> DRSANTNIAVYWGQNSAGTQESLATYCESSDADIFLLSFLNQFPTLGLNFANACSDTFSDGLLHCTQIAEDIETCQSLGKKVLLSLGGASGSYLFSDDSQAETFAQTLWDTFGEGTGASERPFDSAVVDGFDFDIENNNEVGYSALATKLRTLFAEGTKQYYLSAAPQCPYPDASVGDLLENADIDFAFIQFYNNYCSVSGQFNWDTWLTYAQTVSPNKNIKLFLGLPGSASAAGSGYISDTSLLESTIADIASSSSFGGIALWDASQAFSNELNGEPYVEILKNLLTSASQTA

Chitin, a linear polymer of β-(1,4) linked N-acetylglucosamine (GlcNAc) forms the rigid inner layer of the cell wall and is also partially hydrolysed during morphogenesis. This is performed by glycoside hydrolase family 18 (GH18) chitinases that catalyse the cleavage of β-(1,4) glycosidic bonds between GlcNAc residues. In contrast, “plant-type” enzymes are predominantly cell wall associated endochitinases. Here we describe the discovery of novel, low micromolar chemical inhibitors of Aspergillus fumigatus family 18 plant-type chitinase A1 (AfChiA1) by high-throughput screening (HTS).

Exhaustive attempts to obtain a complex of compound 5 with AfChiA1 were unsuccessful. Due to comparable IC50 values between AfChiA1 and ScCTS1 (9.2 μM versus 2.4 μM), as an alternative approach, we selected ScCTS1 as a model to study this interaction. Compound 5 was soaked into ScCTS1 crystals and diffraction data were collected to 1.8 Å. Clear electron density for compound 5 was observed in the active site, corroborating the kinetics data showing that it, like compound 1, is a competitive inhibitor. The ScCTS1–compound 5 complex shows the ligand filling a similar space to that occupied by compound 1 despite the lack of obvious chemical similarities. The dihydroindene moiety inserts into the same pocket as the pyrimidine methyl of compound 1. The hydrogen bonding requirements of the Asp172 side chain (Asp155 in ScCTS1) is satisfied by the linker amine of compound 5, which also donates a potential hydrogen bond to the carboxylate of Glu157 (Glu174 in AfChiA1). Finally the ether oxygen of the ligand accepts a hydrogen bond from the Ala110 backbone (equivalent to Ala124 in AfChiA1). Consequently, the absence of stacking moieties in compound 5 is unusual, though it may help explain the specificity of this molecule for plant-type over bacterial-type family 18 chitinases, as the latter group generally possesses a second tryptophan that forms a ‘lid’ for the active site. Binding of the bulky dihydroindene deep in the ScCTS1 active site induces a conformational change in the protein, with the side chain of Tyr214 (Tyr232 in AfChiA1) and the following loop being pushed out by ∼2 Å compared to the superimposed ScCTS1–acetazolamide complex structure.>[3x]MGQGPELHLASQFVNEACRALVFGGCVEKSSVSRNPEVPFESSAYRIS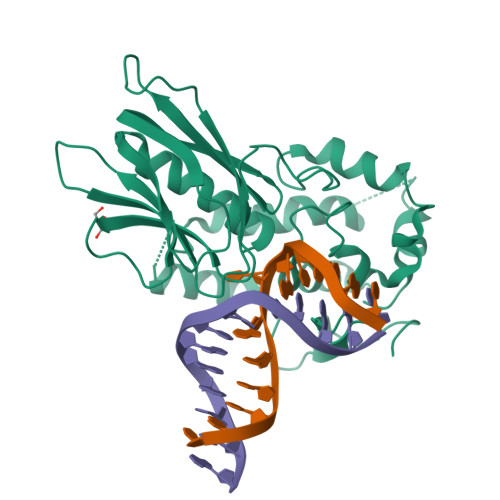ASARGKELRLILSPLPGAQPQQEPLALVFRFGMSGSFQLVPREELPRHAHLRFYTAPPGPRLALCFVDIRRFGRWDLGGKWQPGRGPCVLQEYQQFRENVLRNLADKAFDRPICEALLDQRFFNGIGNYLRAEILYRLKIPPFEKARSVLEALQQHRPSPELTLSQKIRTKLQNPDLLELCHSVPKEVVQLGGKGYGSESGEEDFAAFRAWLRCYGMPGMSSLQDRHGRTIWFQGDPGPLAPKGRKS>GGGRDEHPDARRQAQLRHLLLQDCGSCHGLRLTGGLGPALTPEALRGKPRESLVATVLMGRPQTPMPPWAGLLSADDAGWLVDRLIEGEIAP[11x]

Here, the crystal structure of NirC, a c-type cytochrome co-encoded with other proteins involved in nitrite reduction by the opportunistic pathogen Pseudomonas aeruginosa, has been determined. The iron cation is coordinated by His24 and Met62, which is consistent with mutagenesis studies performed using the orthologue from P. pantotrophus. Whereas NirM is absent in many NirS-producing bacteria and has been assigned to function as an electron transporter for the nitrite reductase, orthologs of NirC are found in nearly all NirS producers, but their function is subject to ongoing discussions.

Because the wild-type protein failed to crystallize, we attempted to reduce the surface entropy by mutating Glu71 to alanine, finally yielding cube-shaped crystals that diffracted anisotropically and possessed a very large orthorhombic unit cell. The crystals diffracted anisotropically to a maximum resolution of 2.12 Å (spherical resolution of 2.83 Å) and initial phases were obtained by Fe-SAD phasing, revealing the presence of 11 NirC chains in the asymmetric unit. Surprisingly, these protomers arrange into one monomer and two different types of 3D domain-swapped dimers, one of which shows pronounced asymmetry. In the three ‘far dimers’ the average iron–iron distance is 28.5 ± 0.2 Å, whereas it is 24.9 ± 0.1 Å in the two ‘close dimers’. In the dimers of NirC observed here, the GloA-score is 0.9 ± 0.2 Å for the far dimers, compared with 3.05 ± 0.01 Å for the close dimers; this is indicative of substantial asymmetry in the latter, which is readily discernible after the superposition of one protomer of a dimer onto the other. In NirC, the increased flexibility leads to antiparallel β-sheet-like interactions of Leu26, Arg27 and Leu28 in the far dimers and no interactions, but with elevated B factors of the hinge loop in the close dimers. Notably, dimerization does not have a major impact on the structure of the heme-binding site, indicating that monomers and dimers could display similar biochemical properties, as has already been found for other N-terminally domain-swapped cytochromes. Importantly, the mutation is not part of the dimer interfaces or the hinge loop, suggesting that it does not cause the simultaneous presence of different NirC oligomeric states observed here. However, the fact that we did not detect dimers even in highly concentrated solutions, together with the observation that crystallization took relatively long and required the introduction of a surface-entropy-reduction mutant that enabled crystal formation through new crystal contacts, currently argues for a crystallization artefact that points towards structural malleability of these proteins rather than a physiological importance of NirC dimers.>GQDLALSCGTSEASADQDKKKWEPDTKFLKTGNSIHATATYQDPSLLSTVPYMTARIFTAPATYEIPIKGDKRHLLRLYFYPSTYTGLNISNSYFTVEANDVTLLSNFSAAITCQALTQAYLVKEYSLAPTDKDVLSIKFTPSDKYRDAFAFINGIEVIQMPELFDTAALVGFTDQTMDAKTANLQSMFRLNVGGQDIPGSQDSGGLTRTWYNDAPYIFSAGLGVTLQASNNFRINYQNMPVSIAPADIYKTARSQGPNGDINLKSNLTWMFQIDKNFTYILRLHFCEFQLSKINQKVFNIYINNRTAQADTTPADIIGWTGEKGIPMYKDYAIYVDANNGGEEITLQMTPSTFGQPEYYDSSLNGLEIFKMDTMKNLAGPNPEPSPMQAEEEVKKEFKNEKRHLEGSENLYFQ[2x]

Members of the plant-specific Catharanthus roseus receptor kinase 1-like (CrRLK1L) family are key players in monitoring the cell-wall status and regulating cell expansion. CrRLK1L family members localize to the plasma membrane and are composed of a cytoplasmic kinase domain, a single transmembrane helix and a variable ligand-binding ectodomain. Loss of FER function impairs pollen-tube reception, whereas ANX1/2, together with BUPS1/2, helps to maintain pollen-tube integrity during polarized tip growth, assuring fertilization. The structures of ANX1 and ANX2 reveal an un­expected novel fold with the two malectin-like domains packed against each other and connected by a short β-hairpin linker, forming a potential ligand-binding cleft.

We obtained crystals for all receptors and diffraction-quality crystals for ANX1 and ANX2. We crystallized ANX1 in space group P1 with two protein molecules per asymmetric unit. We determined the structure of ANX1 via single isomorphous replacement using a platinum derivative. The structures of ANX1 and ANX2 were refined to 1.48 and 1.1 Å resolution, respectively, with residues 26–411 in ANX1 and 28–411 in ANX2 being well defined in electron density. In the case of ANX1 the crystals from both studies were isomorphous (r.m.s.d. of 0.6 Å over 382 corresponding Cα atoms) and grew in similar conditions, with our crystals diffracting to higher resolution (1.48 Å). As CrRLK1Ls have been speculated to bind cell-wall components, we mapped the known carbohydrate-binding sites onto the ANX1 structure. We next explored other potential carbohydrate-binding surfaces: Structural alignment of the bacterial CBM22 (DALI Z-score 8.6) with ANX1 mal-N brings the xylotetraose ligand of CBM22 into close proximity to the distal face of the β-sandwich domain normally used by B-type CBMs for the recognition of carbo­hydrate polymers. We thus tested the binding of ANX1 to various cell-wall-derived carbohydrates of different natures and lengths. We located three and four well defined N-glycans in our high-resolution ANX1 and ANX2 structures, respectively.> TTLLNPYFGEFGGMYVPQILMPALNQLEEAFVRAQKDPEFQAQFADLLKNYAGRPTALTKCQNITAGTRTTLYLKREDLLHGGAHKTNQVLGQALLAKRMGKSEIIAETGAGQHGVASALASALLGLKCRIYMGAKDVERQSPNVFRMRLMGAEVIPVHSGSATLKDACNEALRDWSGSYETAHYMLGTAAGPHPYPTIVREFQRMIGEETKAQILDKEGRLPDAVIACVGGGSNAIGMFADFINDTSVGLIGVEPGGHGIETGEHGAPLKHGRVGIYFGMKAPMMQTADGQIEESYSISAGLDFPSVGPQHAYLNSIGRADYVSITDDEALEAFKTLCRHEGIIPALESSHALAHALKMMREQPEKEQLLVVNLS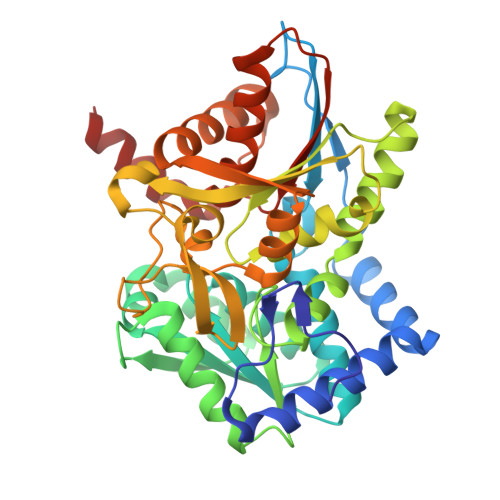GRGDKDIFTVHDILKARGEI>[2x]MGHHHHHHAENLYFQGHMLRLSAPGQLDDDLCLLGDVQVPVFLLRLGEASWALVEGGISRDAELVWADLCRWVADPSQVHYWLITHKHYDHCGLLPYLCPRLPNVQVLASERTCQAWKSESAVRVVERLNRQLLRAEQRLPEACAWDALPVRAVADGEWLELGPRHRLQVIEAHGHSDDHVVFYDVRRRRLFCGDALGEFDEAEGVWRPLVFDDMEAYLESLERLQRLPTLLQLIPGHGGLLRGRLAADGAESAYTECLRLCRRLLWRQSMGESLDELSEELHRAWGGQSVDFLPGELHLGSMRRMLEILSRQALPLD;>[2x]MRNDGGFLLWWDGLRSEMQPIHDSQGVFAVLEKEVRRLGFDYYAYGVRHTIPFTRPKTEVHGTYPKAWLERYQMQNYGAVDPAILNGLRSSEMVVWSDSLFDQSRMLWNEARDWGLCVGATLPIRAPNNLLSVLSVARDQQNISSFEREEIRLRLRCMIELLTQKLTDLEHPMLMSNPVCLSHREREILQWTADGKSSGEIAIILSISESTVNFHHKNIQKKFDAPNKTLAAAYAAALGLI

The majority of traits controlled by rhl transcription factor RhlR depend on PqsE, a dispensable thioesterase in Pseudomonas Quinolone Signal (PQS) biosynthesis that interferes with RhlR through an enigmatic mechanism likely involving direct interaction of both proteins. Here we show that PqsE and RhlR form a 2:2 protein complex that, together with RhlR agonist N-butanoyl-L-homoserine lactone (C4-HSL), solubilizes RhlR and thereby renders the otherwise insoluble transcription factor active. PqsE is a thioesterase that triggers transcription of the RhlR regulon through a hitherto cryptic mechanism, which we identify here as involving a significant chaperone-like component that enhances the stability of RhlR via protein complex formation. In common with many other gram-negative bacteria, two QS circuits use N-acyl-L-homoserine lactones (HSLs) as autoinducers, namely N-(3-oxododecanoyl)-L-HSL (3-oxo-C12-HSL) and N-butanoyl-L-HSL (C4-HSL), which are produced by autoinducer synthases LasI and RhlI and activate the LuxR-type transcription factors LasR and RhlR, respectively.

Interactions between PqsE and RhlR do not involve the autoinducer binding site or the DNA-binding domain (DBD) of RhlR, suggesting that complex formation does not directly interfere with the ability of RhlR to sense C4-HSL and bind to its cognate promoter regions. The homoserine lactone moiety of C4-HSL establishes a hydrogen bond with the side chain of W68, whereas the amide group engages into hydrogen bonds with Y64, D81 and S135. The acyl chain of C4-HSL points into a hydrophobic pocket of the ligand binding site in RhlR, again with high similarity to related structures. The complex is only pseudo-symmetric, i.e. the twofold axes of the PqsE and RhlR proteins are slightly shifted and skewed relative to each other. This leads to the formation of two different contacts between both proteins, one comprising approx. 850 Å2 (contact area 1) and a smaller one involving approx. 310 Å2 (contact area 2) partially overlapping with contact area 1. To validate their relevance, we introduced alanine mutations and investigated their impact on complex formation in E. coli coexpression experiments as well as on pyocyanin production in P. aeruginosa. This revealed the importance of several (e.g. RhlR: D41, E147, E150; PqsE: R150, R170, R172) but not all residues (e.g. RhlR: Q140/Q141; PqsE: R148) within the larger contact area 1, whereas mutation of residues exclusive to contact area 2 had no effect. Notably, only the N-terminus of PqsE is accessible in the complex, explaining why tagging at other termini abrogates complex formation.>[2x]GPGVCKSYKSVALVVGVTGIVGSSLAEVLKLPDTPGGPWKVYGVARRPCPVWLAKKPVEYIQCDVSNNQETISKLSPLKDITHIFYVS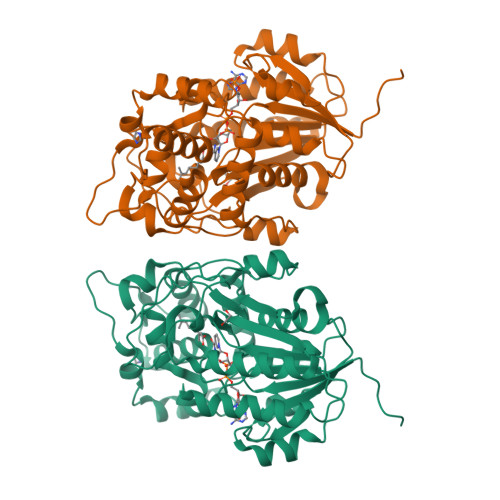WIGSEDCQTNATMFKNILNSVIPNASNLQHVCLQTGIKHYFGIFEEGSKVVPHDSPFTEDLPRLNVPNFYHDLEDILYEETGKNNLTWSVHRPALVFGFSPCSMMNIVSTLCVYATICKHENKALVYPGSKNSWNCYADAVDADLVAEHEIWAAVDPKAKNQVLNCNNGDVFKWKHIWKKLAEEFGIEMVGYVEGKEQVSLAELMKDKDQVWDEIVKKNNLVPTKLKEIAAFWFADIAFCSENLISSMNKSKELGFLGFRNSMKSFVSCIDKMRDYRFIP>[2x]GPDSASRISPGQINQVRPKLPLLKILHAAGAQGEMFTVKEVMHYLGQ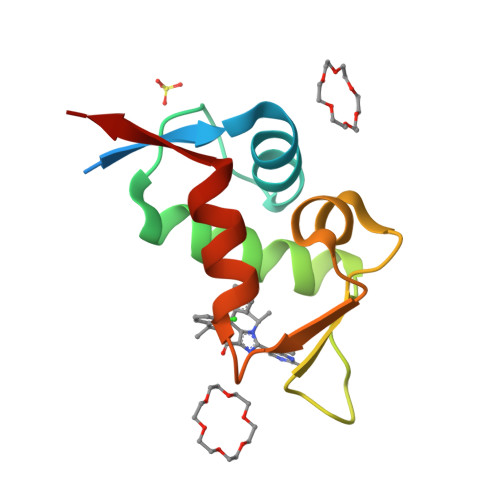YIMVKQLYDQQEQHMVYCGGDLLGELLGRQSFSVKDPSPLYDMLRKNLVTLAT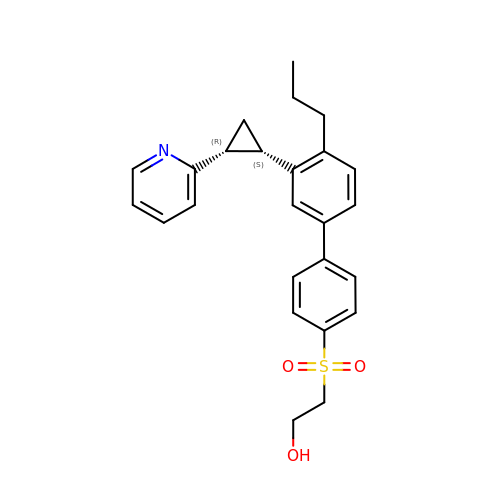2-[4-[4-propyl-3-[(1~{S},2~{R})-2-pyridin-2-ylcyclopropyl]phenyl]phenyl]sulfonylethanol | C25 H27 N O3 S | OOMBYXBTLUCTCM-DNQXCXABSA-N> MSVPAIAPRRKRLADGLSVTQKVFVRSRNGGATKIVREHYLRSDIPCLSRSCTKCPQIVVPDAQNELPKFILSDSPLELSAPI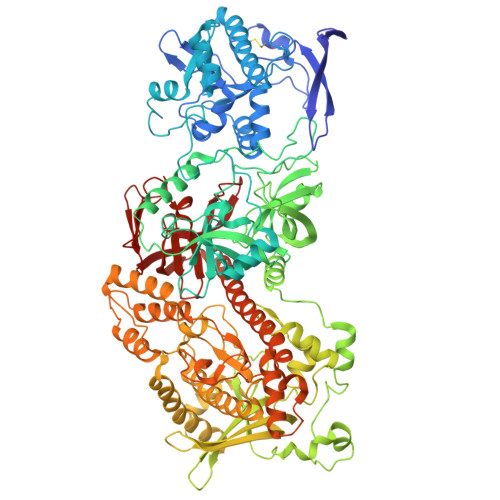GKHYVVLDTNVVLQAIDLLENPNCFFDVIVPQIVLDEVRNKSYPVYTRLRTLCRDSDDHKRFIVFHNEFSEHTFVERLPNETINDRNNRAIRKTCQWYSEHLKPYDINVVLVTNDRLNREAATKEVESNIITKSLVQYIELLPNADDIRDSIPQMDSFDKDLERDTFSDFTFPEYYSTARVMGGLKNGVLYQGNIQISEYNFLEGSVSLPRFSKPVLIVGQKNLNRAFNGDQVIVELLPQSEWKAPSSIVLDSEHFDVNDNPDIEAGDDDDNNESSSNTTVISDKQRRLLAKDAMIAQRSKKIQPTAKVVYIQRRSWRQYVGQLAPSSVDPQSSSTQNVFVILMDKCLPKVRIRTRRAAELLDKRIVISIDSWPTTHKYPLGHFVRDLGTIESAQAETEALLLEHDVEYRPFSKKVLECLPAEGHDWKAPTKLDDPEAVSKDPLLTKRKDLRDKLICSIDPPGCVDINDALHAKKLPNGNWEVGVHIADVTHFVKPGTALDAEGAARGTSVYLVDKRIDMLPMLLGTDLCSLKPYVDRFAFSVIWELDDSANIVNVNFMKSVIRSREAFSYEQAQLRIDDKTQNDELTMGMRALLKLSVKLKQKRLEAGALNLASPEVKVHMDSETSDPNEVEIKKLLATNSLVEEFMLLANISVARKIYDAFPQTAMLRRHAAPPSTNFEILNEMLNTRKNMSISLESSKALADSLDRCVDPEDPYFNTLVRIMSTRCMMAAQYFYSGAYSYPDFRHYGLAVDIYTHFTSPIRRYCDVVAHRQLAGAIGYEPLSLTHRDKNKMDMICRNINRKHRNAQFAGRASIEYYVGQVMRNNESTETGYVIKVFNNGIVVLVPKFGVEGLIRLDNLTEDPNSAAFDEVEYKLTFVPTNSDKPRDVYVFDKVEVQVRSVMDPITSKRKAELLLK> GRFSERAQKVLALSQEEAIRLSHHNIGTEHILLGLIREGEGIAAKALQQLGLGSDKLQKEVEGLVGKGQEGQKSIHSTPHYTP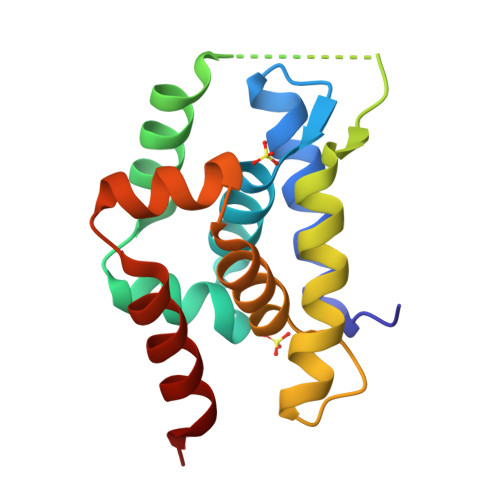RAKKVIELSMDEARKLGHSYVGTEHILLGLIREGEGVAARVLNNLGVSLNKARQQVLQLLGNN> MDAWLQQTVFRGTLSISQGVDDRDLLLAPKWISFLSLSSFLKQKLLSLLRQIRELRLTTTVYPPQDKLMWWSHCCDPEDIKVVILGQDPYHKGQATGLAFSVDPQCQVPPSLRSIFRELEASVPNFSTPSHGCLDSWARQGVLLLNTVLTVEKGRAGSHEGLGWDWFTSFIISSISSKLEHCVFLLWGRKAIDRTPLINAQKHLVLTAQHPSP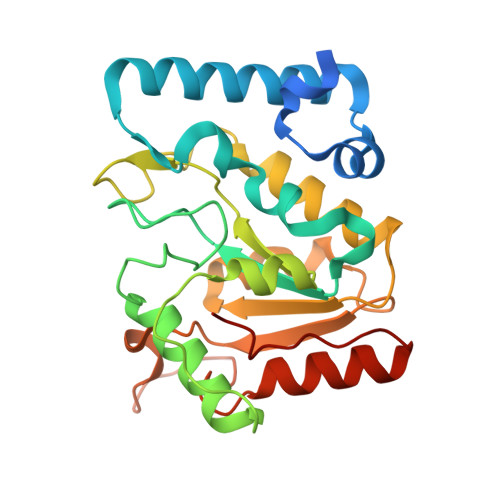LASLGGRHSRWPRFQGCNHFNLANDYLTRHRRETVDWGLLEQ>QENSFTINSVDMKSLPDWTVQNGKQLTLQCFADVSTTSHVKPQHQMLFYKDDVLFYQISSMKSTESYFIPEVRIYDSGTYKCTVIVNNKEKTTAEYQLLVEGVPSPRVTLDKKEAIQGGIVRVQCSVPEEKAPIHFTIEKLELNEKMVKLKREKNSRDQNFVILEFPVEEQDRVLSFRCQARIISGIHMQTSESTK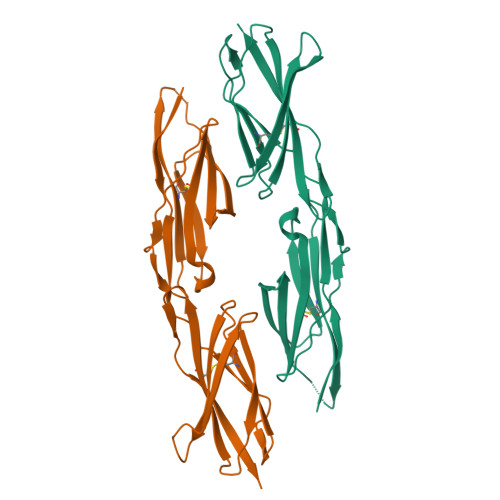SELVTVTESTGHHHHHH[2x]>DYKDDDDKSCLIPENLRNPKKVHENRLPTRAYYYDQDIFESLNGPWAFALFDAPLDAPDAKNLDWETAKKWSTISVPSHWELQEDWKYGKPIYTNVQYPIPIDIPNPPTVNPTGVYARTFELDSKSIESFEHRLRFEGVDNCYELYVNGQYVGFNKGSRNGAEFDIQKYVSEGENLVVVKVFKWSDSTYIEDQDQWWLSGIYRDVSLLKLPKKAHIEDVRVTTTFVDSQYQDAELSVKVDVQGSSYDHINFTLYEPEDGSKVYDASSLLNEENGNTTFSTKEFISFSTKKNEETAFKINVKAPEHWTAENPTLYKYQLDLIGSDGSVIQSIKHHVGFRQVELKDGNITVNGKDILFRGVNRHDHHPRFGRAVPLDFVVRDLILMKKFNINAVRNSHYPNHPKVYDLFDKLGFWVIDEADLETHGVQEPFNRHTNLEAEYPDT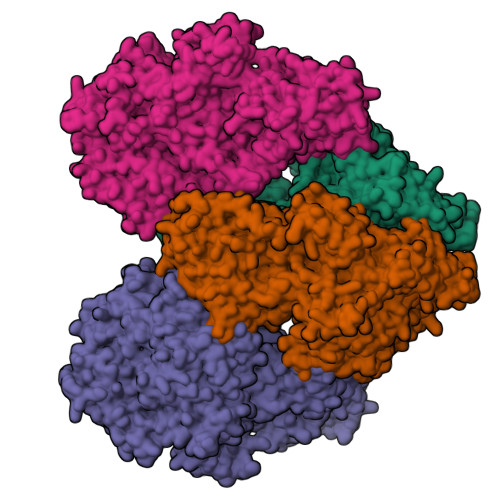KNKLYDVNAHYLSDNPEYEVAYLDRASQLVLRDVNHPSIIIWSLGNEACYGRNHKAMYKLIKQLDPTRLVHYEGDLNALSADIFSFMYPTFEIMERWRKNHTDENGKFEKPLILCEYGHAMGNGPGSLKEYQELFYKEKFYQGGFIWEWANHGIEFEDVSTADGKLHKAYAYGGDFKEEVHDGVFIMDGLCNSEHNPTPGLVEYKKVIEPVHIKIAHGSVTITNKHDFITTDHLLFIDKDTGKTIDVPSLKPEESVTIPSDTTYVVAVLKDDAGVLKAGHEIAWGQAELPLKVPDFVTETAEKAAKINDGKRYVSVESSGLHFILDKLLGKIESLKVKGKEISSKFEGSSITFWRPPTNNDEPRDFKNWKKYNIDLMKQNIHGVSVEKGSNGSLAVVTVNSRISPVVFYYGFETVQKYTIFANKINLNTSMKLTGEYQPPDFPRVGYEFWLGDSYESFEWLGRGPGESYPDKKESQRFGLYDSKDVEEFVYDYPQENGNHTDTHFLNIKFEGAGKLSIFQKEKPFNFKISDEYGVDEAAHACDVKRYGRHYLRLDHAIHGVGSEACGPAVLDQYRLKAQDFNFEFDLAFE[4x]The RNA recognition motif (RRM) binds to nucleic acids as well as proteins. Here we describe the mode of interaction between hnRNP L and LL with the methyltransferase SETD2. We demonstrate that for the interaction to occur, a leucine pair within a highly conserved stretch of SETD2 insert their side chains in hydrophobic pockets formed by hnRNP L RRM2. Notably, the SETD2 binding region in RRM2 is distinct from its RNA-binding interface.

The conserved 30 amino acid sequence of the SHI domain did not reveal any clues as to how it might engage hnRNP L. Hence, to further explore the molecular basis of this interaction, we determined the crystal structure of hnRNP L RRM2 in complex with the SETD22167–2192 peptide at 1.80 Å resolution. There are two complexes contained in a crystallographic asymmetric unit, with hnRNP L RRM2 chains A and C associating with SETD22167–2192 chains B and D, respectively. The hnRNP L RRM2 in the complex adopts a β1α1β2β3α2β4β5 conformation that forms a five-stranded β sheet packed against two α-helices. When bound to hnRNP L RRM2, SETD22167–2192 adopts a U-shaped conformation contacting the RRM dorsal helical face. Although all residues of the SETD22167–2192 peptide could be clearly traced, only a fraction at the C-terminus of this peptide (2183NAGKVLLPTP2192) was found to directly contact the RRM, burying ~477 Å of the solvent-exposed area of hnRNP L RRM2. In detail, the bulk side chain of SETD2Leu2188 is accommodated by a hydrophobic pocket which is lined by hnRNP LLeu251 from α2, hnRNP LIle214 from α1, hnRNP LIle256 from the α2-β4 loop, and hnRNP LLeu263 from β4. In addition, the side chain of SETD2Leu2189 stretches into a neighboring shallow apolar depression lined by hnRNP L Ile214, Val210, Ile256, and Tyr257. Furthermore, the residues downstream of the Leu pair, including 2190-Pro-Thr-Pro-2192, together with SETD2Leu2189, wrap around the hnRNP LTyr257 and hnRNP LTyr204, providing further binding affinity and specificity. Notably, hnRNP LTyr257 makes van der Waals contacts with both SETD2Leu2189 and SETD2Pro2192, playing an important role in hnRNP L-SETD2 interaction. Although the N-terminus of the SETD22167–2192 does not interact with the RRM2 directly, we found that the residues from substantial van der Waals and hydrogen contact with the C-terminus of the SETD2 peptide, possibly helping to fix the conformation of the peptide and thus, enhance the binding.

>HHHHHHMDDSRSVNSVLLFTILNPIYSITTDVLYTICNPCGPVQRIVIFRKNGVQAMVEFDSVQSAQRAKASLNGADIYSGCCTLKIEYAKPTRLNVFKNDQDTWDYTNPN[2x];>[2x]YPPGYPMQAYVDPSNPNAGKVLLPTP> MHYELSAAARAAFLSKYRDFPHYMENRNFTPPKDGGMWLRFNYIEGDTLYLSIDRKCKSYIAIVQIGVVFPPGSGVDEARLKAKEIADFFKDG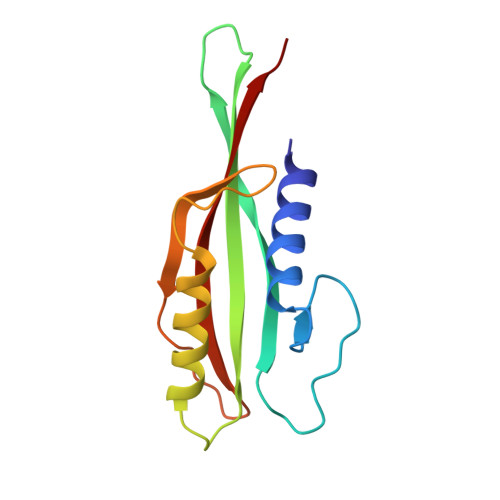KMLNVGYIFEGAIVHQIVKHESGWMIPVRFTVRVDTKET>[6x]EKDPLWLYKVLLTKGIEVWFDIKLEKYGIKRNNRVDYIAKSSLQQIVFEIIGKTPKNIAVPTYIGAYEPSKPEKWEEEGIKYINLFKPTPLMKVKPVKEMPEIVKNLLLNLFDYDAKSMGLFINWLAFIYQYKERTGVAWIFMGKQGTGKGLLVDLLKKIFEEHMSSNITDA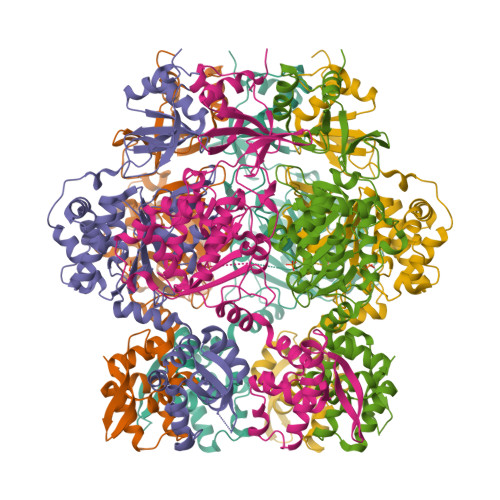NLDSQFNPYLYNKLIVHLNEVSADNRKSRMLVKNRLKTWITDETLYINRKNMKEVEIKNFCNFIINSNETIPVDIEDSDRRFNVIECNNVLKEQEWWTTESYQEILNNAEGFAKYLAGIKVDRSKVNEVVMSEKKKAIVETTESVLKQIAKALTDRDIEWFLDNGLEGVVEKNIVNDFQWEELQEAITTGVIPNKYLMIIVEQILGDSKTITWIKRNIITPYQVGETTVVKMAGKPIRAIVVG Due to the amphipathic property, S1P cannot diffuse freely but has to be transported across the cell membrane through active transport. Among these transporters, Spns2 is the first identified and the most extensively studied. Human Spns2 is a classical MFS member with twelve transmembrane (TM) helices and a molecular weight of ~58 kDa, which is small for cryo-EM analysis. Here, we reported two cryo-electron microscopy (EM) structures of human Spns2 in inward-open conformations bound to S1P or inhibitor 16d.

Previously, the Webster group reported an S1P analog 16d as an Spns2 competitive inhibitor. Here, we determined the WT Spns2 structure (named Spns2wt, without PGS fusion) bound with the inhibitor 16d (IC50 = 1.93 μM) using cryo-EM at an overall resolution of 3.5 Å. The structure of Spns2wt also adopted an inward-open conformation, which is almost identical to the Spns2fusion structure. Although the density for inhibitor 16d is discontinuous and challenging for model building, we roughly estimated that inhibitor 16d occupied the S1P binding pocket. Moreover, we could only measure its inhibition for S1P transport in the cell-based efflux assay when we overexpressed Spns2 without adding exogenous Sph in the medium. We speculated that the high concentration of exogenous S1P will cover up the Spns2 inhibition by 16d, consistent with the reported weak binding efficacy.

> MHHHHHHHHHHSGDEVDAGSGHMMCLECASAAAGGAEEEEADAERRRRRRGAQRGAGGSGCCGARGAGGAGVSAAGDEVQTLSGSVRRAPTGPPGTPGTPGCAATAKGPGAQQPKPASLGRGRGAAAAILSLGNVLNYLDRYTVAGVLLDIQQHFGVKDRGAGLLQSVFICSFMVAAPIFGYLGDRFNRKVILSCGIFFWSAVTFSSSFIPQQYFWLLVLSRGLVGIGEASYSTIAPTIIGDLFTKNTRTLMLSVFYFAIPLGSGLGYITGSSVKQAAGDWHWALRVSPVLGMITGTLILILVPATKRGHADQLGDQLKARTSWLRDMKALIRNRSYVFSSLATSAVSFATGALGMWIPLYLHRAQVVQKTAETCNSPPCGAKDSLIFGAITCFTGFLGVVTGAGATRWCRLKTQRADPLVCAVGMLGSAIFICLIFVAAKSSIVGAYICIFVGETLLFSNWAITADILMYVVIPTRRATAVALQSFTSHLLGDAGSPYLIGFISDLIRQSTKDSPLWEFLSLGYALMLCPFVVVLGGMFFLATALFFVSDRARAEQQVNQLAMPPASVKV> MEAGYAEIAAVQFNIAGDNDHKRQGVMEVTISNLFEGTLPAEGGIYDARMGTTDHHYKCITCSHQRKQCMGHPGILQMHAPVLQPLFIAEIRRWLRVICLNCGAPIVDLKRYEHLIRPKRLIEAASSQTEGKQCYVCKAVHPKIVKDSEDYFTFWADQQGKIDKLYPQIIREIFSRVTYDTVVKLGRSKNSHPEKLVLKAIQIPPISIRPGIRLGIGSGPQSFHDINNVIQYLVRKNLLIPKDLQIVRGQKIPLNIDRNLQTIQQLYYNFLLDSVSTTATQGGTGKRGIVMGARPAPSIMRRLPRKEGRIRKSLLGSQVWSISRSTICGNSDLHLDEVGYPISFARTLQVAETVQHYNINRLMPYFLNGKRQYPGCSRVYKQITQSVHDIEGLKQDFRLEVGDILYRDVVTGDVAFFNRQPSLERSSIGVHRIVVLENPKISTFQMNVSACAWYNADFDGDQMNLWVPWSVMSRVEAELLCSVRNWFISTKSSGPVNGQVQDSTVGSFLLTRTNTPMGKNVMNKLHAMGLFQTTQTDPPCFANYSPTDLLDGKSVVSMLLRQTPINYQRAPTWYSEVYAPYMHYNKQDISTQIRNGELIEGVLDKKAVGAGSSGGIYHLISRRYGPQQALKMIFATQQLALNYVRNAGFTVSTADMLLTPEAHQEVQEIINELLLESEEINNRLLHGDIMPPIGLTTHDFYEKLQLNALKFPDRILKPIMNSINPETNGLFQMVATGAKGSNPNMIHIMAGIGQIEINTQRIQPQFSFGRTLVYYPRFALEAQAYGFICNSYIAGLTSPEFIFGEMNGRFDLINKALSTSSTGYANRKAIFGLQSCIVDYYRRVSIDTRLVQQLYGEDGLDARQLETVRFETIMLSDQELEDKFKYTGIQSPLFEEEFSRLKKDRDKYRQIFLNVENFNFSQLLTDVRQVPVNVASIVKNILLSSTSGVLPFDEKSILQKYAMVKTFCKNLPYVFINNIQERLQTPIPVYLKRAASLMRMLIRIELATVKTLNITCEQMSAILDLIRLQYTQSLINYGEAVGILAAQSVSEPLTQYMLDSHHR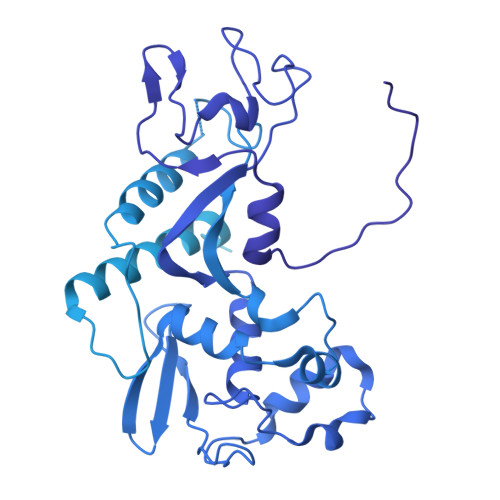SVAGGTNKSGIVRPQEIFSAKPVEAEQSSEMLLRLKNPEVETNKTYAQEIANSIELITFERLILQWHLLYETYSSTKKNVMYPDFASDVEWMTDFLENHPLLQPPEDIANWCIRLELNKTTMILKSISLESIINSLRAKHPNTYIMHSVENTASGIPIIIRIYLRESAFRRSTNTRMATDEKIAVNVVDKLLNSTIRGIPGIKNANVVKLMRHRVDAQGKLVRLDNIYAIKTNGTNIFGAMLDDNIDPYTIVSSSIGDTMELYGIEAARQKIISEIRTVMGDKGPNHRHLLMYADLMTRTGQVTSLEKAGLNAREPSNVLLRMALSSPVQVLTDAAVDSAVNPIYGIAAPTLMGSVPRIGTMYSDIIMDEKYITENYKSVDSLIDML>[8x]SNAMPQQKNFVTMPAQHQNKQPGIESLMNPLPQFEDPNYKGSEKLKGKNVLITGGDSGIGRAVSIAFAKEGANIAIAYLD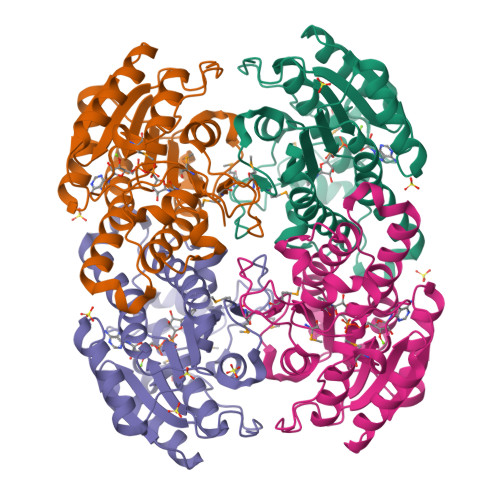EEGDANETKQYVEKEGVKCVLLPGDLSDEQHCKDIVQETVRQLGSLNILVNNVAQQYPQQGLEYITAEQLEKTFRINIFSYFHVTKAALSHLKQGDVIINTASIVAYEGNETLIDYSATKGAIVAFTRSLSQSLVQKGIRVNGVAPGPIWTPLIPSSFDEKKVSQFGSNVPMQRPGQPYELAPAYVYLASSDSSYVTGQMIHVNGGVIVNG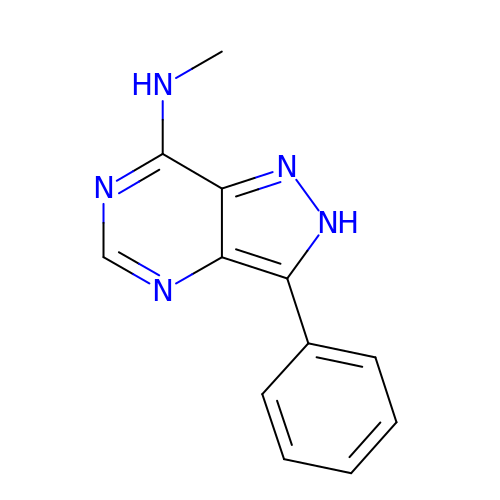~{N}-methyl-3-phenyl-2~{H}-pyrazolo[4,3-d]pyrimidin-7-amine | C12 H11 N5 | XIEMFNUUOUPBSW-UHFFFAOYSA-N>[4x]MHHHHHHLPNITILATGGTIAGGGDSATKSNYTVGKVGVENLVNAVPQLKDIANVKGEQVVNIG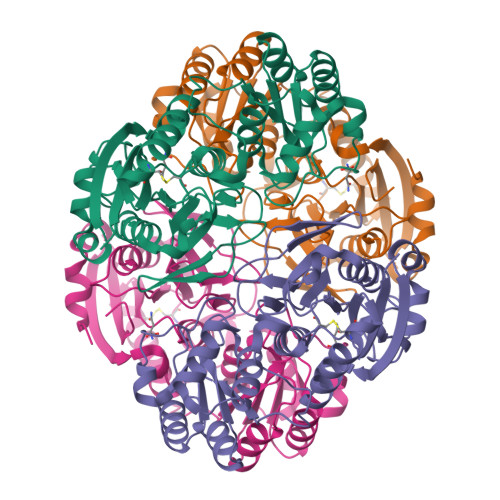SQDMNDNVWLTLAKKINTDCDKTDGFVITHGVDTMEETAYFLDLTVKCDKPVVMVGAMRPSTSMSADGPFNLYNAVVTAADKASANRGVLVVMNDTVLDGRDVTTTNTTDVATFKSVNYGPLGYIHNGKIDYQRTPARKHTSDTPFDVSKLNELPKVGIVYNYANASDLPAKALVDAGYDGIVSAGVGNGNLYKSVFDTLATAAKTGTAVVRSSRVPTGATTQDAEVDDAKYGFVASGTLNPQKARVLLQLALTQTKDPQQIQQIFNQY> SHMLRLSAPGQLDDDLCLLGDVQVPVFLLRLGEASWALVEGGISRDAELVWADLCRWVADPSQVHYWLITHKHYDHCGLLPYLCPRLPNVQVLASERTCQAWKSESAVRVVERLNRQLLRAEQRLPEACAWDALPVRAVADGEWLELGPRHRLQVIEAHGHSDDHVVFYDVRRRRLFCGDALGEFDEAEGVWRPLVFDDMEAYLESLERLQRLPTLLQLIPGHG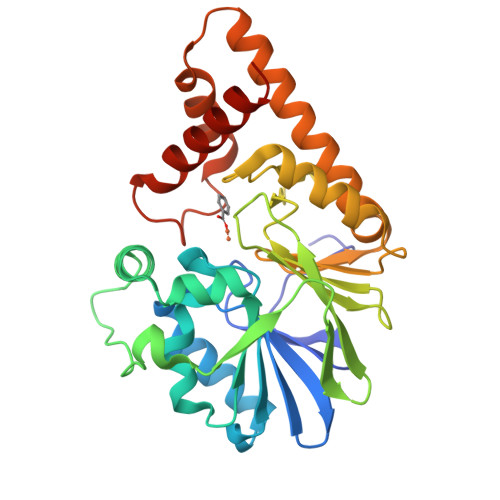GLLRGRLAADGAESAYTECLRLCRRLLWRQSMGESLDELSEELHRAWGGQSVDFLPGELHLGSMRRMLEILSRQALPLD(quinolin-2-ylmethyl)phosphonic acid | C10 H10 N O3 P | 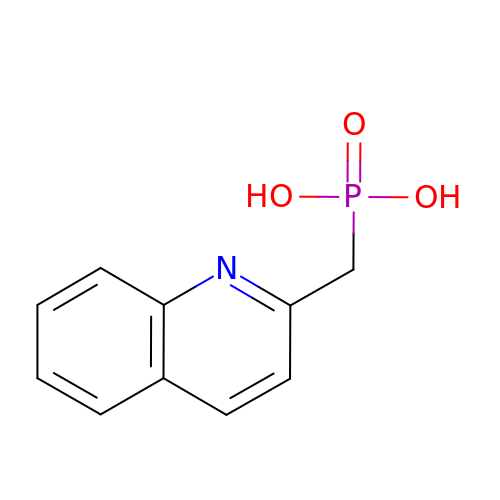SZCYKKWPKXABPU-UHFFFAOYSA-N> GPGSDLPPKV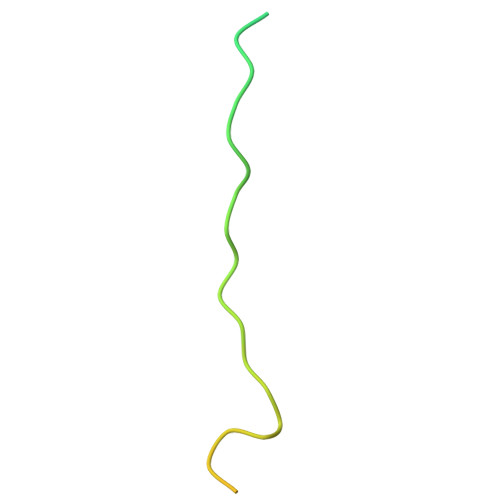VPSKQLLHSDHMEMEPETMETKSVTDYFSKLHMGSVAYSCTSEFHHHHHH>MGSSHHHHHHMIRKVLVANRGEIAVRIIRACQELGIRTVVAYSTADRDSLAVRLADEAVCIGPPPAAKSYLNAPALISAALVSGCDAIHPGYGFLSENPYFAEMCADCKLTFIGPPPEPIRLMGDKAIGRETMRKAGVPTVPGSDGEVRSLEEAIDVARQIGYPVLLKPSGGGGGRGMRVAYDEADLQRAFPTARAEAEAAFGNGALLLEKYLTRVRHVEIQVLADQYGHAIHLGERDCSAQRRHQKIVEEAPSPAVTPELRERMGADAVRGIKSIGYVNAGTLEFLLDQDGNYYFI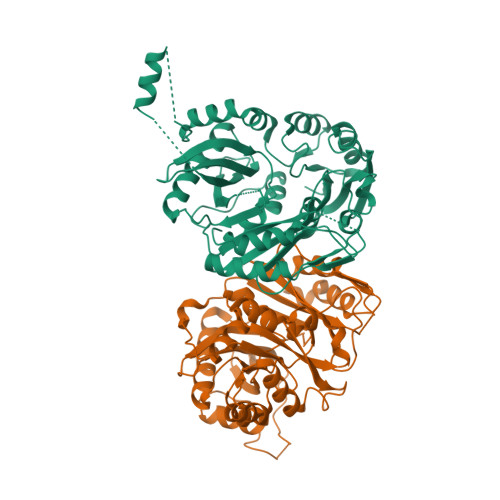EMNTRIQVEHPVTEQVTGIDLVRWQLLIASGERLTLRQEDIKITRHAIECRINAEDPERDFLPASGEVEFYLPPGGPGVRVDSHLYSGYTPPGTYDSLLAKIITFGDTRDEALNRMRRALNECVITGIKTTIPFQLALIDDPEFRAGRIHTGYVAELLRQWKETLNPV[2x]Aromatic residues cluster in the core of folded proteins, where they stabilize the structure through multiple interactions. NMR studies in the 1970s demonstrated that aromatic side chains can undergo ring flips—that is, 180° rotations of the χ2 dihedral angle (Cβ–Cγ axis)—even when engaged in stabilizing interactions in the hydrophobic core. Here we capture ring flipping events of a buried tyrosine residue in the SH3 domain of the JNK-interacting protein 1 (JIP1). Our data therefore suggest that the conformation of the aromatic ring at position 526 is determined by steric interactions dictated by the size of the surrounding amino acids.

The SH3 domain of JIP1 undergoes exchange between two distinct conformations, as evidenced by 15N NMR relaxation measured at multiple temperatures (Supplementary Discussion). The 15N and 1HN relaxation dispersion data were analysed simultaneously according to a two-site exchange model in which a highly populated major state interconverts with a low-populated minor state (Supplementary Discussion). The analysis of the data gives a population of the minor state of pminor = 2.8 ± 0.1% and an exchange rate constant of kEX = 2,600 ± 70 s−1. Aromatic 1H–13C heteronuclear single quantum coherence (HSQC) spectra show averaging of the NMR signals of the tyrosine ε1/ε2 nuclei of Y526, which shows that full 180° ring flipping occurs. During the structural transition between the major and the minor state, a void volume is created around the ring of Y526 that corresponds to a pocket expansion of 65 Å3; this is mainly due to the structural reorganization of the side chain of Q520. Notably, the transition from the eclipsed, major conformation to the staggered, minor conformation is associated with a structural change from a rare, classic β-bulge to a common, canonical β-strand conformation. Breathing motions along the structural trajectory between the major and the minor state generate the necessary void volume for fast ring flipping of Y526 to take place.

>[4x]GHMEQTHRAIFRFVPRHEDELELEVDDPLLVELQAEDYWYEAYNMRTGARGVFPAYYAIEVTK>GPSGQEVPWLSSVRYGTVEDLLAFANHISNTAKHFYGQRPQESGILLNMVITPQNGRYQIDSDVLLIPWKLTYRNIGSDFIPRGAFGKVYLAQDIKTKKRMACKLIPVDQFKPSDVEIQACFRHENIAELYGAVLWGETVHLFMEAGEGGSVLEKLESCGPMREFEIIWVTKHVLKGLDFLHSKKVIHHDIKPSNIVFMSTKAVLVDFGLSVQMTEDVYFPKDLRGTEIYMSPEVILCRGHSTKADIYSLGATLIHMQTGTPPWVKRYPRSAYPSYLYIIHKQAPPLEDIADDC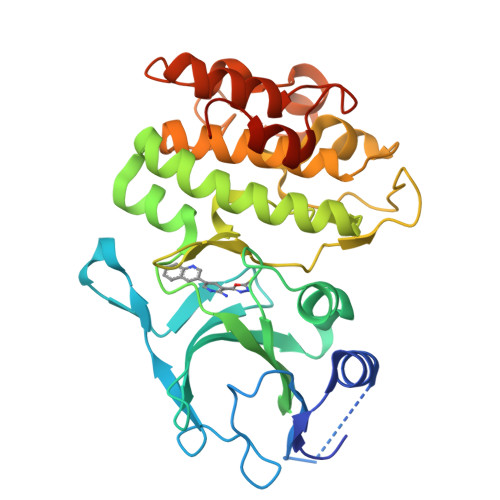SPGMRELIEASLERNPNHRPRAADLLKHEALNPPREDQ[3x]(3-exo)-8,8-dimethyl-3-(4-{[(1-methyl-2-oxo-1,2-dihydroquinolin-4-yl)oxy]methyl}-1H-1,2,3-triazol-1-yl)-8-azoniabicyclo[3.2.1]octane 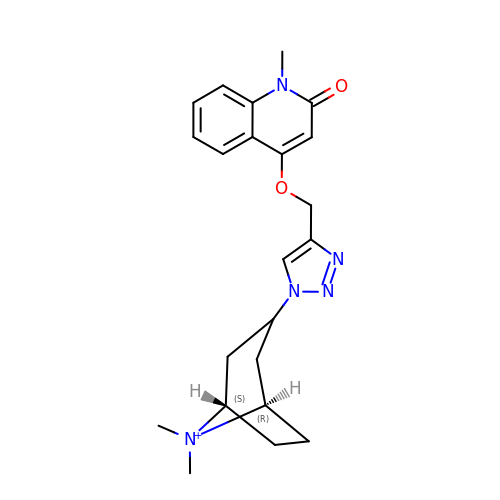| C22 H28 N5 O2 | YGBMUEMPFNRGJC-NNZMDNLPSA-N(2~{R},4~{R},5~{R},6~{R})-6-[(1~{R})-1,2-bis(oxidanyl)ethyl]-4,5-bis(oxidanyl)oxane-2-carboxylic acid | C8 H14 O7 | 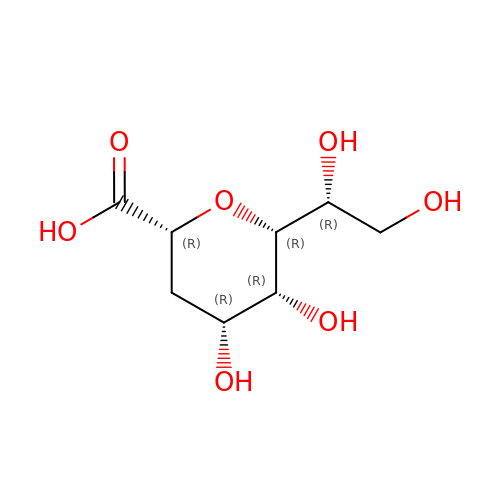ANWKOKWAJKGXFO-NYMZXIIRSA-N> MPYIEKLELKGFKSYGNRKVVIPFSKGFTAIVGANGSGKSNIGDAILFVLGGLSAKAMRATRISDLIFAGSKGEPPAKYAEVAIYFNNEDRGFPIDEDEVVIKRRVYPDGRSAYWLNGRRATRSEILDLLSAAMISPEGYNLVLQGDITKFIKMSPLERRQLIDEISGIAEYDAKKEKALEELKQAEENLARVDLLIKEVKKQLDKLEKERNDALRYLDLKERLERARVALLLGEIKRLESMIDEGERKRAEIESGGSENTIKVKSAQLRIQLEEKRRELKHFDAALIRSVKEVSLDLEVLRKEIEDMEAEIKALEPVNMKAIEDFEVVERRYLELKSKREKLEAEKESIIEFINEIEKEKKNVFMRTLEAIAKNFSELFAKLSPGGSARLILENPEDPFSGGLEIEAKPAGKDVKRIEAMSGGEKALTALAFIFAIQRFKPAPFYLFDEIDAHLDDANVKRVADLIKESSRESQFI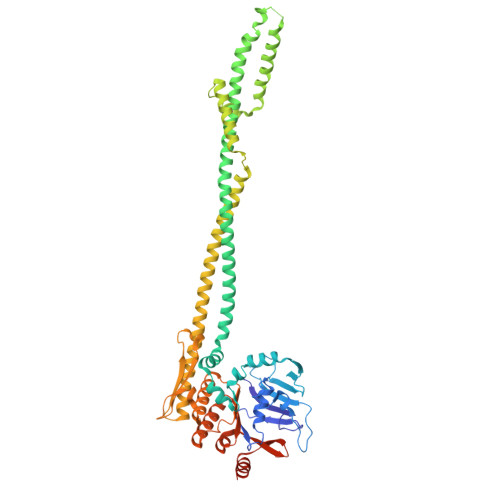VITLRDVMMANADKIIGVSMRDGVSRVVSLSLEKAMKILEEAKKRNEATIGGVDAGSSSRPGL>MADFKFEPMRSLIYVDCVSEDYRPKLQRWIYKVHIPDSISQFEPYVTKYAFYPSFPIPPQGDRFGYARMQLTEHHWLVSDLDPRLEIKAIAETFPMDVLVWQGQIPAAAHTDAQIDSDGDAGNAARKSNNAEGNPFIFAFLPMWWEKDLKGKGRTIEDGANYRFNMTIGFPEGVDKAEGEKWLFE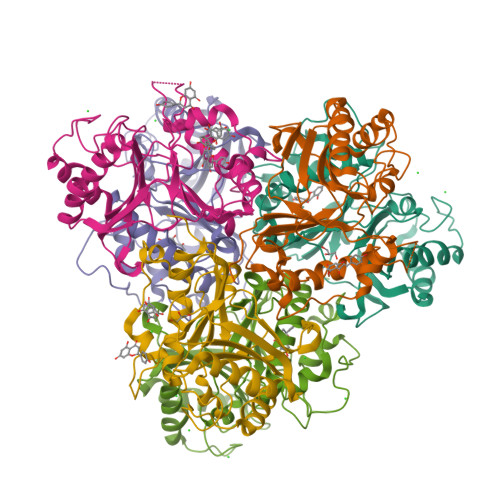KVVPILQAAPECTRVLASAVKKDINGCVMDWVLEIWFENQSGWYKVMVDDMKALEKPSWAQQDAFPFLKPYHNVCSAAVADYTPSNNLANYRGYITMR[6x]> SELNEKLATAWEGFTKGDWQNEVNVRDFIQKNYTPYEGDESFLAGATEATTTLWDKVMEGVKLENRTHAPVDFDTAVASTITSHDAGYINKQLEKIVGLQTEAPLKRALIPFGGIKMIEGSCKAYNRELDPMIKKIFTEYRKTHNQGVFDVYTPDILRCRKSGVLTGLPDAYGRGRIIGDYRRVALYGIDYLMKDKLAQFTSLQADLENGVNLEQ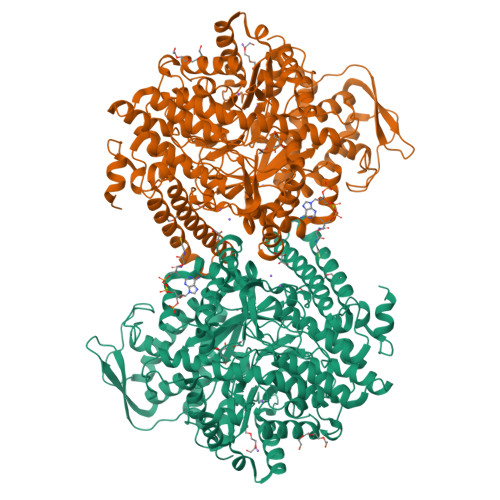TIRLREEIAEQHRALGQMKEMAAKYGYDISGPATNAQEAIQWTYFGYLAAVKSQNGAAMSFGRTSTFLDVYIERDLKAGKITEQEAQEMVDHLVMKLRMVRFLRTPEYDELFSGDPIWATESIGGMGLDGRTLVTKNSFRFLNTLYTMGPSPEPNMTILWSEKLPLNFKKFAAKVSIDTSSLQYENDDLMRPDFNNDDYAIACCVSPMIVGKQMQFFGARANLAKTMLYAINGGVDEKLKMQVGPKSEPIKGDVLNYDEVMERMDHFMDWLAKQYITALNIIHYMHDKYSYEASLMALHDRDVIRTMACGIAGLSVAADSLSAIKYAKVKPIRDEDGLAIDFEIEGEYPQFGNNDPRVDDLAVDLVERFMKKIQKLHTYRDAIPTQSVLTITSNVVYGKKTGNTPDGRRAGAPFGPGANPMHGRDQKGAVASLTSVAKLPFAYAKDGISYTFSIVPNALGKDDEVRKTNLAGLMDGYFHHEASIEGGQHLNVNVMNREMLLDAMENPEKYPQLTIRVSGYAVRFNSLTKEQQQDVITRTFTQSM> TPEVGELIEKVRKAHQETFPALCQLGKYTTNNSSEQRVSLDIDLWDKFSELSTKCIIKTVEFAKQLPGFTTLTIADQIT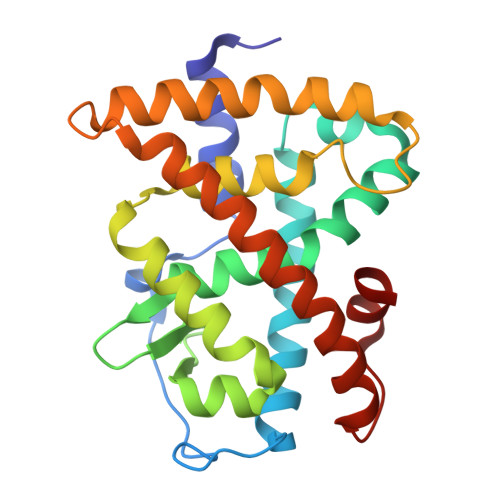LLKAACLDILILRICTRYTPEQDTMTFSDGLTLNRTQMHNAGFGPLTDLVFAFANQLLPLEMDDAETGLLSAICLICGDRQDLEQPDRVDMLQEPLLEALKVYVRKRRPSRPHMFPKMLMKITDLRSISAKGAERVITLKMEIPGSMPPLIQEMLE>[2x]SMDEECVLEAENKKLVEDQEKLKTELRKTSDALSKAQNDVMEMKMQSER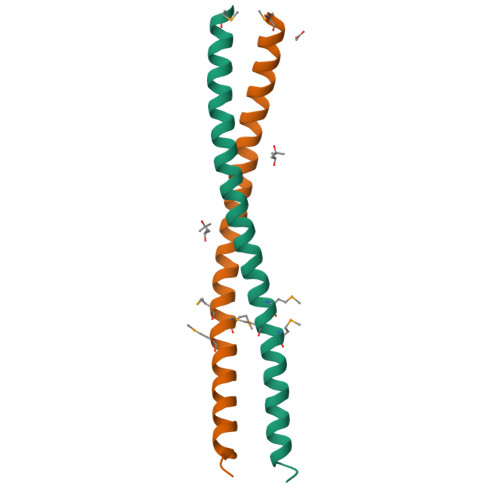LSKEYDQLLKEHSEL4-[3-(4,5-dihydro-1,2-oxazol-3-yl)-2-methyl-4-methylsulfonyl-phenyl]carbonyl-2-methyl-1~{H}-pyrazol-3-one 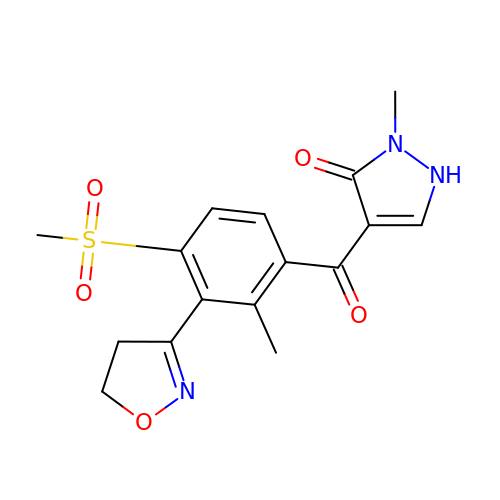| C16 H17 N3 O5 S | BPPVUXSMLBXYGG-UHFFFAOYSA-N>SNAFLDYGLSEADPDVHAIINKEKDRQFRSLELIASENFTSKAVMEAVGSCLTNKYSEGLPGKRYYGGNEHIDELEILCQQRALAAFHLDGDKWGVNVQPLSGSPANFAVYTAILKPHDRIMGLDLPHGGHLSHGFMTAKRRVSGTSIYFESMPYRLDESTGVIDYDMLEKTAALFRPKLIIAGASAYPRDIDYARFRKIADSVGAFLMMDMAHVSGLIAASVLADPFEFVDIVTTTTHKSLRGPRGGMIFFKKDAVHGVDLESAINNAVFPGLQGGPHNHTIGGLAVCLKYAQSPDFKNYQNQVVANCRALANRLVEHEYKLVSGGSDNHLVLVDLRPSGIDGARVEKILDMASITLNKNSVPGDKSALVPGGIRIGSPAMTTR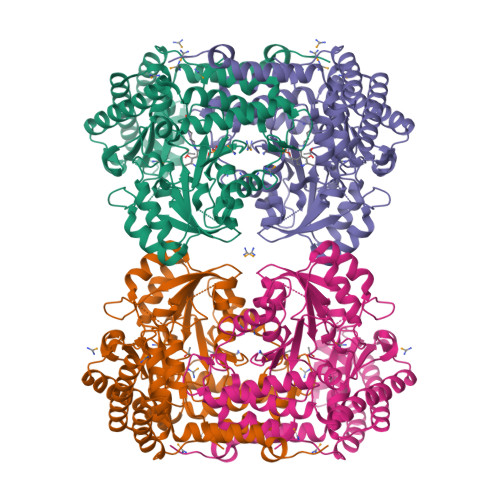GLGEKEFELIADLIHEGVRISLEAKSLVSGTKVQDFLNFVLAPEFPLGDKVSNLRRKVEALATQYPIPGV[2x]> ASGSSGMSIVSLLGIKVLNNPAKFTDPYEFEITFECLESLKHDLEWKL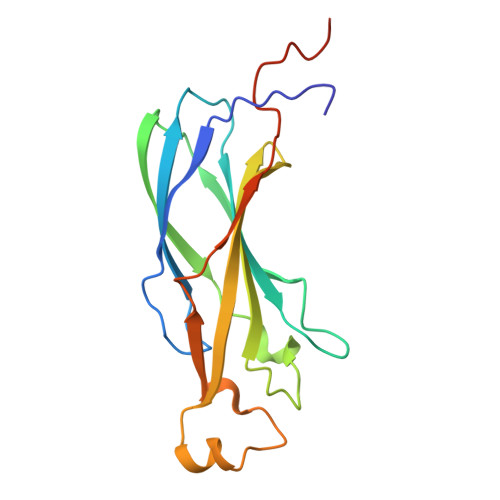TYVGSSRSLDHDQELDSILVGPVPVGVNKFVFSADPPSAELIPASELVSVTVILLSCSYDGREFVRVGYYVNNEYDEEELRENPPAKVQVDHIVRNILAEKPRVTRFNIVWDNENEGDLYPPEQPGV>[2x]ALEEVVRYLGPHNEIPLTLTRDSETGHFLLKHFLPILQQYHDTGNINETNPDSFPTDEERNKLLA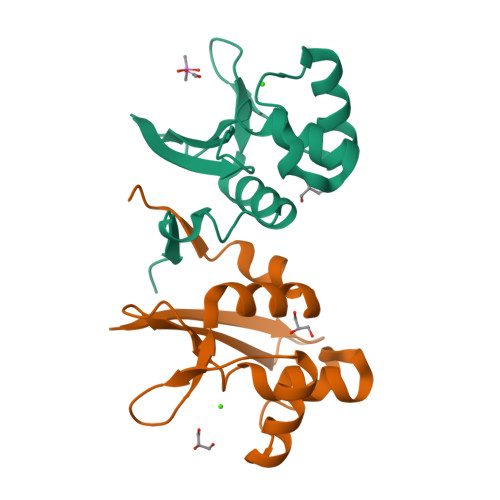HYGIAVNTDDRGELWIELEKCLQLLNMLNLFGLFQDAFEFEEPETDQDEEDPSHSKLPEN>[8x]GSEELLDLFNRQVTQEFTASQVYLSASIWFDQNDWEGMAAYMLAQSAEEREHGLGFVDFANKRNIPIELQAVPAPVSCAEWSSPEDVWQSILELEQANTRSLLNLAEAASTCHDFAVMAFLNPFHLQQVNEEDKIGSILAKVTDENRTPGLLRSLDVVSFLGPCLFRSV

Ferritin from the marine pennate diatom Pseudo-nitzschia multiseries (PmFTN) plays a key role in sustaining growth in iron-limited ocean environments. Typically formed from 24 subunits arranged as a symmetric, hollow sphere, ferritins take up soluble Fe2+ and catalyze its oxidation, with the resulting Fe3+ being stored as an oxy-hydroxide mineral in its central cavity. The di-iron catalytic ferroxidase center of PmFTN (sites A and B) has a nearby third iron site (site C) in an arrangement typically observed in prokaryotic ferritins. Here we demonstrate that Glu-44, a site C ligand, and Glu-130, a residue that bridges iron bound at sites B and C, limit the rate of post-oxidation reorganization of iron coordination and the rate at which Fe3+ exits the ferroxidase center for storage within the mineral core.

To explore the role of site C in iron mineralization by PmFTN, Glu-44 was substituted with glutamine and histidine, residues that occur naturally at this position in other characterized ferritins. Three crystal structures were obtained from E44Q PmFTN crystals soaked for 5 min (E44Q Fe (5 min)), 45 min (E44Q Fe (45 min)), and overnight (E44Q Fe (o.n.)) in an aerobic Fe2+ solution. Reducing the Fe2+ exposure time of crystals to 5 and 45 min resulted in iron bound at sites A and B at lower occupancy, with the inclusion of Asn-97 in the coordination sphere for Fe-B. Site C remained unoccupied (data not shown). Iron was not found within the B-channels in structures from crystals with shorter soak durations. Substitution of Glu-44 with glutamine resulted in the loss of iron binding at site C in iron soaking experiments. In the E44Q variant, this rearrangement occurs ∼75-fold more rapidly than in the wild type protein (and ∼30-fold more rapidly than in the E130A variant). The overall mineralization kinetics for E44Q PmFTN showed that this enhancement does not translate into a large increase in the rate of overall core formation.> MKKYIYIYFFFITITINDLVINNTSKCVSIERRKNNAYINYGIGYNGPDNKITKSRRCKRIKLCKKDLIDIGAIKKPINVAIFGSTGSIGTNALNIIRECNKIENVFNVKALYVNKSVNELYEQAREFLPEYLCIHDKSVYEELKELVKNIKDYKPIILCGDEGMKEICSSNSIDKIVIGIDSFQGLYSTMYAIMNNKIVALANKESIVSAGFFLKKLLNIHKNAKIIPVDSEHSAIFQCLDNNKVLKTKCL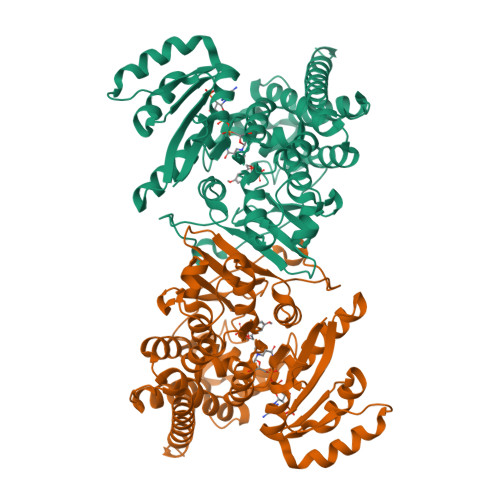QDNFSKINNINKIFLCSSGGPFQNLTMDELKNVTSENALKHPKWKMGKKITIDSATMMNKGLEVIETHFLFDVDYNDIEVIVHKECIIHSCVEFIDKSVISQMYYPDMQIPILYSLTWPDRIKTNLKPLDLAQVSTLTFHKPSLEHFPCIKLAYQAGIKGNFYPTVLNASNEIANNLFLNNKIKYFDISSIISQVLESFNSQKVSENSEDLMKQILQIHSWAKDKATDIYNKHNSS Recent studies have identified a dsDNA deaminase from Burkholderia cenocepacia, DddA, an interbacterial toxin that is delivered to contacting cells by the type VI secretion system and mediates antagonism between Gram-negative bacteria. However, unlike APOBECs that only deaminate ssDNA, DddA selectively deaminates cytosines in dsDNA. Interestingly, DddA shares a strong preference for the 5′-TC target sequence with A3A, A3B and several other APOBEC family members. The crystal structures show that DddA engages the minor groove of a sharply bent dsDNA.

To understand how DddA interacts with dsDNA substrates, we crystallized the toxin domain (Gly1290 to Pro1422) of B. cenocepacia DddA in complex with a 14-base pair (bp) dsDNA substrate containing the 5′-TC target sequence. DddA with a substitution of the catalytically essential glutamic acid residue (E1347A) was used to capture the enzyme–substrate complex. The structure of the DddA–dsDNA complex was determined in two different crystal forms and refined to 2.39 and 2.62 Å resolution, respectively. The structures obtained in the two crystal forms are very similar overall, with a root mean square deviation (r.m.s.d.) of 1.37 Å for all protein and DNA atoms, and of 0.45 Å for the protein backbone atoms, although they differ in the conformation of the target 2′-deoxycytidine nucleotide. In the structure with the cytosine base parked in the DNA major groove, Glu1370 side chain is pointed away from the DNA. DddA Phe1375 intercalates in dsDNA and displaces the 5′ (−1) thymine, which in turn replaces the target cytosine and forms a noncanonical T–G base pair with the juxtaposed guanine. This tandem displacement mechanism allows DddA to locate a target cytosine without flipping it into the active site. The DddA–dsDNA structure trapped with the target cytosine parked in the major groove suggests that DddA can locate 5′-TC motifs in double-stranded DNA without engaging the cytosine base in the active site. It may represent an intermediate conformation that allows DddA to scan through a DNA sequence to locate target cytosines.

> GSYALGPYQISAPQLPAYNGQTVGTFYYVNDAGGLESKVFSSGGPTPYPNYANAGHVAGQSALFMRDNGISEGLVFHNNPEGTCGFCVNMTETLLPENAKMTVVPPEGAIPVKRGATGETKVFTGNSNSPKSPHHHHHH>[3x]MVVVAAFEGWNDAGDAAGDAVAHLAASWQALPIVEIDDEAYYDYQVNRPVIRQVDGVTRELQWPAMRISHCRPPGSDRDVVLMCGVEPNMRWRTFCDELLAVIDKLNVDTVVILGALLADTPHTRPVPVSGAAYSAASARQFGL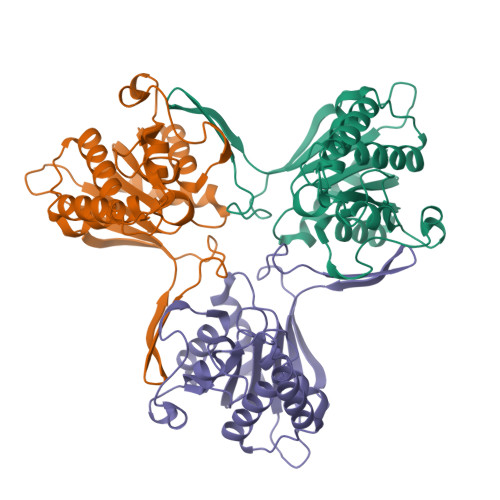QETRYEGPTGIAGVFQSACVGAGIPAVTFWAAVPHYVSHPPNPKATIALLRRVEDVLDVEVPLADLPAQAEAWEREITETIAEDHELAEYVQTLEQHGDAAHHHHHH>DSVYVQNPQIPILVDRTDNVLFRIRIPDATKGDVLNRLTIRFGNEDKLSEVKAVRLFYAGTEAATKGRSRFAPVTYVSSHNIRNTRSANPSYSIRQDEVTTVANTLTLKTRQPMVKGINYFWVSVEMDRNTSLLSKLTSTVTEVVINDKPAVIAGEQAAVRRMGIGVRHAGDDGSASFRIPGLVTTNKGTLLGVYDVRYNNSVDLQEHIDV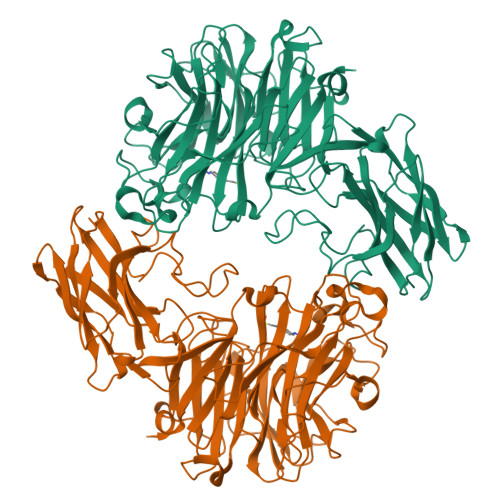GLSRSTDKGQTWEPMRIAMSFGETDGLPSGQNGVGDPSILVDERTNTVWVVAAWTHGMGNARAWTNSMPGMTPDETAQLMMVKSTDDGRTWSESTNITSQVKDPSWCFLLQGPGRGITMRDGTLVFPIQFIDSLRVPHAGIMYSKDRGETWHIHQPARTNTTEAQVAEVEPGVLMLNMRDNRGGSRAVSITRDLGKSWTEHSSNRSALPESICMASLISVKAKDNIIGKDLLLFSNPNTTEGRHHITIKASLDGGVTWLPAHQVLLDEEDGWGYSCLSMIDRETVGIFYESSVAHMTFQAVKIKDLIR[2x]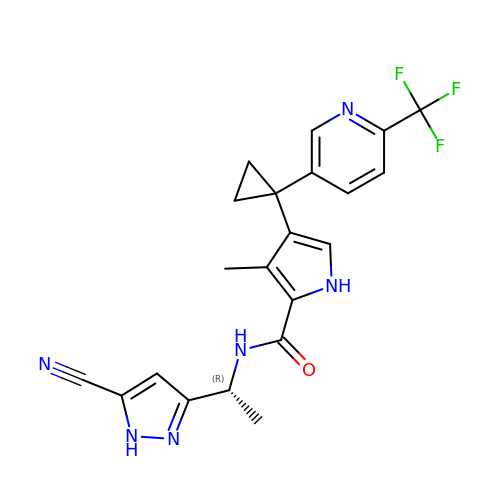N-[(1R)-1-(5-cyano-1H-pyrazol-3-yl)ethyl]-3-methyl-4-{1-[6-(trifluoromethyl)pyridin-3-yl]cyclopropyl}-1H-pyrrole-2-carboxamide | C21 H19 F3 N6 O | POQZTSJDTKESSW-GFCCVEGCSA-N> QAQITGRPEWIWLALGTALMGLGTLYFLVKGMGVSDPDAKKFYAITTLVPAIAFTMYLSMLLGYGLTMVPFGGE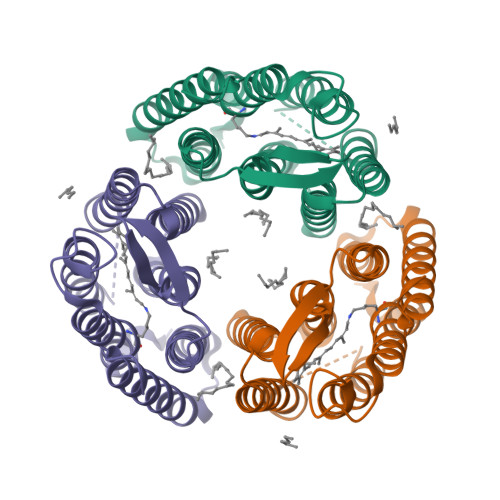QNPIYWARYADWLFTTPLLLLDLALLVDADQGTILALVGADGIMIGTGLVGALTKVYSYRFVWWAISTAAMLYILYVLFFGFTSKAESMRPEVASTFKVLRNVTVVLWSAYPVVWLIGSEGAGIVPLNIETLLFMVLDVSAKVGFGLILLRSRAIFG> GSHM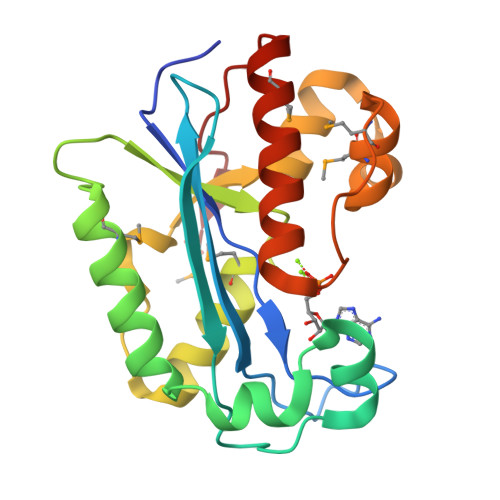ADSYYDYICIIDFEATCEEGNPPEFVHEIIEFPVVLLNTHTLEIEDTFQQYVRPEINTQLSDFCISLTGITQDQVDRADTFPQVLKKVIDWMKLKELGTKYKYSLLTDGSWDMSKFLNIQCQLSRLKYPPFAKKWINIRKSYGNFYKVPRSQTKLTIMLEKLGMDYDGRPHCGLDDSKNIARIAVRMLQDGCELRINEKM Here, we address this challenge by presenting the results of our comprehensive and systematic investigation of Upstream of N-Ras (Unr), an RBP with multiple RBDs and a model system for understanding sequence specificity of modular RBDs toward target RNAs. In Drosophila, Unr (dUnr) performs sex-specific roles during dosage compensation. In female flies, dUnr, together with Sex-lethal (Sxl), represses translation of Male-specific lethal 2 (Msl2), the rate-limiting component of the dosage compensation complex (DCC) (Abaza and Gebauer, 2008; Abaza et al., 2006; Duncan et al., 2006), whereas in male flies, dUnr has an opposite role and acts together with the RNA helicase Maleless (Mle) presumably as an RNA chaperone to remodel the lncRNA roX2 (RNA on X 2), which promotes the assembly of the DCC (Militti et al., 2014). Although reported to contain five ssRNA-binding cold-shock domains (CSDs), we demonstrate that Unr includes an additional four CSDs that do not bind RNA (pseudo-RBDs) but are involved in mediating RNA tertiary structure specificity by reducing the conformational heterogeneity of Unr.

In the crystal structure of CSD456, interdomain contacts between CSD5 and both ncCSD4 and ncCSD6 are clearly discernable and mediated by F477 on ncCSD4; L505, T521, R533, Q538, E547, L549, and R582 on CSD5; and F593, N663, and R662 on ncCSD6. These contacts appear to keep the domains at a certain distance and orientation to each other. The fit between experimentally observed scattering densities and back-calculated scattering densities from the crystal structure (χ of 1.02; SASBDB: SASDHJ7) strongly suggests that the fixed domain arrangement seen in the crystal structure is maintained in solution. Also, electron density in the corresponding region in ncCSD4 and ncCSD6 was weak or absent in X-ray diffraction data of CSD456, indicating flexibility. CSD456, featuring only one canonical CSD, binds with a KD of 16 μM, comparable with the affinity of CSD1 alone (Hennig et al., 2014a). Similar observations were made for CSD456, where ncCSD4 and ncCSD6 flanking CSD5 do not show major CSPs. We focused our analysis on interdomain residues located in loop regions that lack secondary structure, yet were identified to form interdomain contacts. We generated a series of single mutants as shown in Figure 4A, as well as double and triple mutants as follows: F477A/R582A (referred to as 45 ID given that it disrupts interdomain interactions between CSDs 4 and 5), Q538A/F593A (56 ID, disrupting CSDs 5 and 6 interactions), and L803A/Y865A/I887A (78 ID, disrupting CSDs 7 and 8 interface). Overall, CSD456 and CSD78 mutants displayed decreased stability when compared with wild-type (WT) CSD456 and CSD78, as established by measuring melting temperatures using differential scanning fluorimetry (DSF).

> GGAVDSTVYKGQVLKSLDRNNPVRQNNDPLPGRIRYRALDYSEVEVPFGDKDQKGDFTLRHGDWVQFLLATDRRDQLQRATSIALLDETFKVSGEKREQGTIASLKEGFGFLRCVERQARLFFHFTEVLDTSREIDINDEVEFTVIQEPGLAYNNSRLQAIRIKHLPPNSVQFETLVASNIEGCVTREAPKSPIKSQDRVEGGVITYEHADVKKTIMYFLKDCEKPPRIGERVRFDIYMVKRNKECIAVNVQQVSLH O-tert-butyl-N-[(9H-fluoren-9-ylmethoxy)carbonyl]-L-threonyl-N-{(2R)-5-ethoxy-5-oxo-1-[(3S)-2-oxopyrrolidin-3-yl]pentan-2-yl}-L-phenylalaninamide 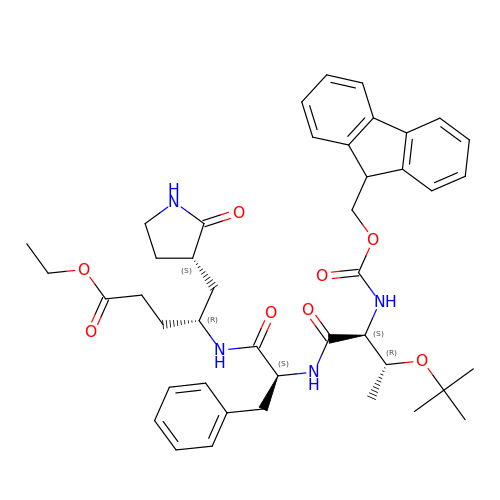| C43 H54 N4 O8 | KZMJRFUAZFUTII-YAPRVMGASA-N> NSTNDDDSIGTRWAVLIA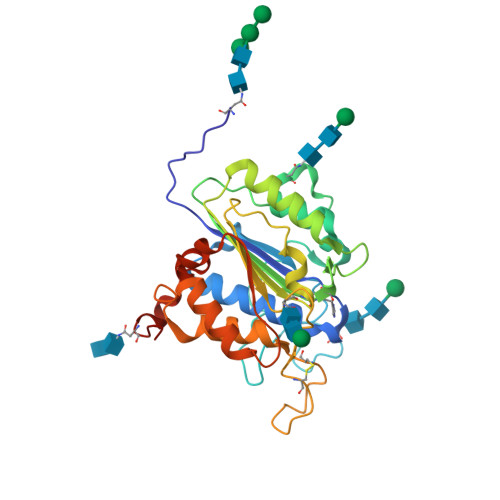GSKGYHNYRHQADVCHMYQILRKGGVKDENIIVFMYDDIAYNESNPFPGIIINKPGGENVYKGVPKDYTGEDINNVNFLAAILGNKSAIIGGSGKVLDTSPNDHIFIYYAXGAPGKIGMPSKPYLYADDLVDTLKQKAATGTYKSMVFYVEAANAGSMFEGLLPEGTNIYAMAASNSTEGSWITYCPGTPDFPPEFDVCLGDLWSITFLEDCDAHNLRTETVHQQFELVKKKIAYASTVSQYGDIPISKDSLSVYMGTDPANDNRTFVDEN> MTSAQQPTPFAVRSNVPRGPHPQQERSIKTRAQILEAASEIFASRGYRGASVKDVAERVGMTKGAVYFHFPSKESLAIAVVEEHYARWPAAMEEIRIQGFTPLETVEEMLHRAAQAFRDDPVMQAGARLQSERASIDAELPLPYVDWTHLLEVPLQDAREAGQLRAGVDPAAAARSLVAAFFGMQHVSDNLHQRADIME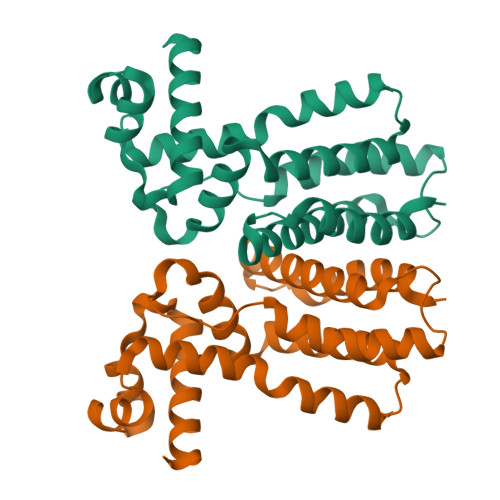RWQELRELMFFALRA We recently characterized two novel HSL family esterases from the thermophilic fungus Rhizomucor miehei: RmEstA and RmEstB. The physiological substrates of RmEstA and RmEstB detected in our studies have been found to be short-chain triacylglycerol, linalyl acetate, and butyl butyrate. Both of these enzymes belong to the α/β hydrolases and exhibit distinct substrate specificities: RmEstA shows highest activity toward longer-chain esters, whereas RmEstB favors hydrolysis of shorter-chain esters. The three-dimensional structures of two HSL esterases from R. miehei, RmEstA and RmEstB, were determined. Both of the esterases were composed of a core catalytic domain and a cap domain, exhibiting the typical α/β-hydrolase fold. A classical catalytic triad consisting of Ser161 (Ser164 in RmEstB) as the nucleophile, His292 (His291 in RmEstB) as the proton acceptor/donor, and Asp262 (Asp261 in RmEstB) as the residue stabilizing the His was identified in RmEstA (RmEstB).

The crystal structures of RmEstA and RmEstB were determined at 2.41 Å and 2.27 Å resolutions, respectively. The monoclinic space group of RmEstB was C121 with four molecules in the asymmetric unit. The four monomers were arranged as two canonical dimers to further form a tetramer via hydrogen bonding network. The substrate-binding pocket of RmEstB extended ∼11 Å from the protein surface to the catalytic residue Ser164. This deep hydrophobic cleft was funnel-shaped and surrounded by four α-helices (α1, α2, α6, and α8) and the loop regions (His88–Gly91 and Ile290–Ala297). The substrate-binding pocket of RmEstB is funnel-shaped with ∼11 Å from the protein surface to the catalytic residue Ser164, a distance that just fits the acyl chains of substrates with carbon chain lengths shorter than C4. Esters with acyl chain lengths longer than C4 therefore hardly bind to the substrate-binding site due to steric hindrance. The structural differences between the substrate-binding pockets of the two esterases suggest that several aromatic residues (Phe222 and Trp92) block the substrate-binding pocket in RmEstB, which might contribute to the restriction in carbon chain lengths of the ester substrates. Phe222 and Trp92 are located in the center of the substrate-binding pocket, close together (4.1 Å). Structural comparison and mutagenesis analysis in the present study indicated that the side chains of residues in the substrate-binding pocket create a steric hindrance, thereby potentially altering substrate specificity in the esterases; moreover, residue Phe222 played a vital role in RmEstB’s variation in substrate specificity.

>[4x]MAPTVKLKPYCQNIADAATIDSTQYPPEVVRKAEAASIIDDPKALEGLPDVYLEEKTINRKNGSKIELTITRPLDTENQVLPPIVFFHGGGWVVGSKLTHRRTVYELTVRARAAVIFVNYSLSPEVRFPTALEECLDAVVWVAKEENAKSINVDPTKLVVAGDSAGGNLSAVVCIRAKQLGLNIIKGQVLIYPVTDDNFETDSYKQFAENYYLTRKLMVWFFDHYIPDKKDRQSIFACPLKASIDDLRVLPRALVITAEADVLREEGEAYARKLIEAGNDVTAVRYLGIIHGIFNLATLSPTGSEILDHIVAWLQKTWKLEHHHHHH FLAVIOLIN | C10 H6 O5 | 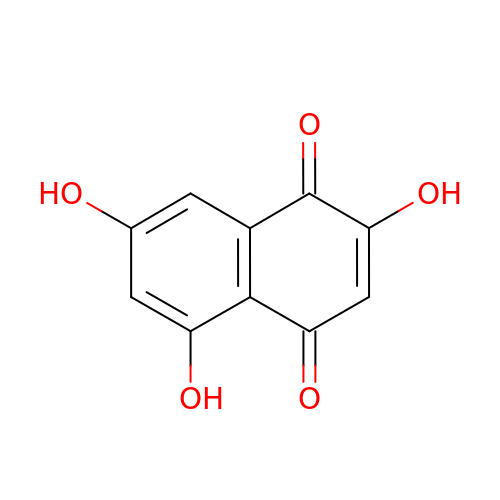RROPNRTUMVVUED-UHFFFAOYSA-N> SVYELQVQKSVTVQEGLCVLVPCSFSYPWRSWYSSPPLYVYWFRDGEIPYYAEVVATNNPDRRVKPETQGRFRLLGDVQKKNCSLSIGDARMEDTGSYFFRVERGRDVKYSYQQNKLNLEVTALIEKPDIHFLEPLESGRPTRLSCSLPGSCEAGPPLTFSWTGNALSPLDPETTRSSELTLTPRPEDHGTNLTCQMKRQGAQVTT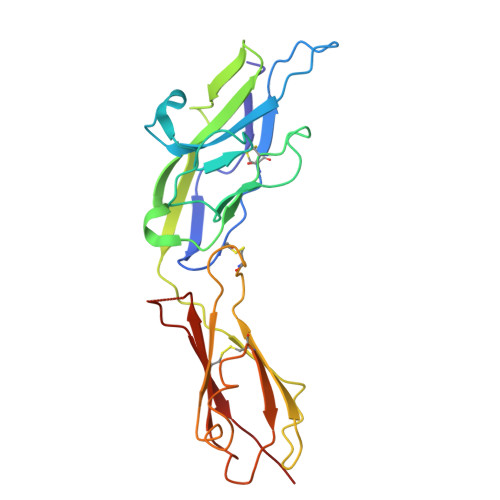ERTVQLNVSL> MFRRAIPLLSANIPRSVWDPAQHNPNWSDSYGHDITNRRAWPARKWTVGLEPCTPREWLQFSHRNLAYAYNGALRACHSLPSMLLLYKEMKQRGVKVDVDTMNVLLTRAARHEHIQVDDVFLLFDELVALGARPDLAAAETLHTVLSHSASMPEEWREARRLQLVELYNNLAMEEVERLAPHRADRLLKEQMKRFRGNLQQLGSGLRPTVYCRYLHTTHTAAVLLEEVHNFLWELVPNDHPAMEIPALQLRVPFVASVLRRPSVNPGVSLASVSRAEFGDTDVCAVFLAAAERMVDADFDDQRPVSE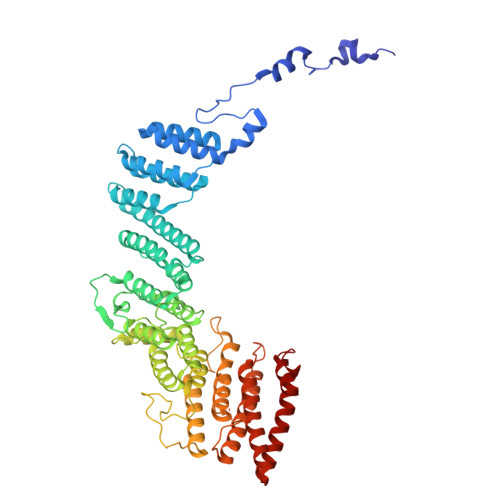RRLFLSLLTMISYSGVLYTSDLMAQLMEMVKYSNNDETRDSDAQRVLRYALRGSSAAQDSASRTLWHSVEKVADCRVVGRYIGARNPWNPIRVCFDEQGVFKAYPISTTTTTREVSPPEGNGAVTQEQRASCVEGRTLEALNMRWDDVRRLIECTGVLVTPPSERCPQQQKMEVFTGMAVYLRTVATGRRYEGGEDVLSDGAVATSSCEQRRRGTLFAEGYDFDVWVRLFSLVQEVRHDMEKFMADHTLQCVEPEFECWEALLVTLRCALDFCVVQMQGGGARGTEREVVERLFRDVVALREELIEESRTRFGGRMRVLWLQEA> SNAMNPTFHADKPIYSQISDWMKKQMI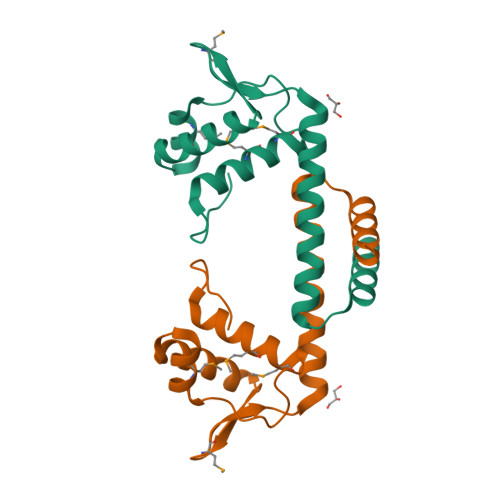TGEWKGEDKLPSVREMGVKLAVNPNTVSRAYQELERAGYIYAKRGMGSFVTSDKALFDQLKKELADAITERFLEEAKSIGLDDQTAIELLIKRSRNHE>SMGRKVTVATCALNQWALDFEGNLQRILKSIEIAKNRGARYRLGPELEICGYGCWDHYYESDTLLHSFQVLAALLESPVTQDIICDVGMPVMHRNVRYNCRVIFLNRKILLIRPKMALANEGNYRELRWFTPWSRSRHTEEYFLPRMIQDLTKQETVPFGDAVLVTWDTCIGSEICEELWTPHSPHIDMGLDGVEIITNASGSHHVLRKANTRVDLVTMVTSKNGGIYLLANQKGCDGDRLYYDGCAMIAMNGSVFAQGSQFSLDDVEVLTATLDLEDVRSYRAEISSRNLAASRASPYPRVKVDFALSCHEDLLAPISEPIEWKYHSPEEEISLGPACWLWDFLRRSQQAGFLLPLSGGVDSAATACLIYSMCCQVCEAVRSGNEEVLADVRTIVNQISYTPQDPRDLCGRILTTCYMASKNSSQETCTRARELAQQIGSHHISLNIDPAVKAVMGIFSLVTGKSPLFAAHGGSSRENLALQNVQARIRMVLAYLFAQLSLWSRGVHGGLLVLGSANVDESLLGYLTKYDCSSADINPIGGISKTDLRAFVQFCIQRFQLPALQSILLAPATAELEPLADGQVSQTDEEDMGMTYAELSVYGKLRKVAKMGPYSMFCKLLGMWRHICTPRQVADKVKRFFSKYSMNRHKMTTLTPAYHAENYSPEDNRFDLRPFLYNTSWPWQFRCIENQVLQLERAEPQSLDGVD[2x]

NAD+ synthetase can be either monofunctional ammonia-dependent NAD+ synthetase using uniquely free ammonia as a substrate or multifunctional glutamine-dependent NAD+ synthetase (glnNAD+ synthetase) using glutamine as the source of ammonia. glnNAD+ synthetase catalyzes the ATP-dependent formation of NAD+ from nicotinic acid adenine dinucleotide (NaAD+) at the synthetase domain using the ammonia generated from the glutaminase domain21. Here, we report the structural and kinetic characterizations of hsNadE and a direct structural comparison of the closed and active conformation of (1) hsNadE structure in complex with a synthetase intermediate analog at 2.84 Å resolution and (2) tbNadE structure in complex with glutamine, sulfonamide derivative 1 (5′-O-(N-(nicotinyl)sulfamoyl) adenosine; SFI), and PPi at 3.14 Å resolution. Both structures are snapshots of the enzymes in the allosteric state with the synthetase active site loop ordered revealing an exclusive rearrangement of the glutaminase active site and the molecular tunnels.

We co-crystalized wild type hsNadE with NaAD+ and AMP (the synthetase intermediate analog), and MgPPi, which activates the glutaminase activity in hsNadE by 12-fold, to obtain the crystal structure of the hsNadE in the closed conformation of the synthetase active site and with the activated glutaminase active site. The co-crystals of hsNadE crystallized in needle-like shape diffracted up to 2.84 Å resolution. Two molecules are present in the asymmetric unit as a homodimer, whereas a tetramer was found in tbNadE structure. Analysis with the Caver program reveals an intra-subunit tunnel forming within a chain in hsNadE structure unlike the inter-subunit tunnel found in tbNadE. The ammonia tunnel is also sealed off at both ends and the glutamine-binding pocket is inaccessible in hsNadE. In the ATP-binding site of hsNadE, AMP and MgPPi are bound in a deep cleft as reported in the tbNadE structure 27 with one Mg ion coordinated to three O atoms of PPi, to the main chains of ATP-binding site residues including Val360HS and Asp361HS (ATP pyrophosphate fingerprint), and a Cl− atom (red sphere). In this hsNadE complex, the ATP-binding site is fully protected by the closure of the P2 loop via three crucial contacts with the ligands and with the synthetase residues. In the absence of a ligand at the glutaminase active site of hsNadE complex, the Glu176HS side chain moves 78° towards the Cys175HS–Glu45HS–Lys114HS triad compared to the herein described tbNadE complex and the other previously reported complexes. In addition, this conformation of the Glu176HS side chain blocks the glutamine tunnel and clashes with the glutamine molecule as shown in the overlay with the tbNadE–glutamine–SFI–PPi structure. Interestingly, in hsNadE Trp179HS-subunit A is observed in a conformation that restricts the entrance to the glutamine tunnel, and Glu176HS is positioned to prevent glutamine binding.>MALLNFQKPDKVIMIDSTDFEGKFEFRPLEPGYGLTVGNALRRVLLSSLEGFAITSVRIDGVEHEFSVVPGVVEDVTEIILNLKQVRFKRQIDDVESETVSISVSGKEQLTAGDFQKFISGYQVLNPDLVICNMGPKVSINMEIVIEKGRGYVPAEENKKSNAPLGSIAVDSVYTPVKNVKYSIENYRVEQKTDYEKLVFEIITDGSIHPKDALTEAAKVLIHHFMLFSDERITLEADEIAQTETYDEESLHMRQLLKTKLVDMDLSVRALNCLKAAEVDTLGDLVSFNKNDLMKFRNFGKKSLTELEELVINKGLQFGMDLSKYKLDKD[2x];> MFTNTIERVNFASAKNIPEYPDFLDIQIKSFQDFFQLETKSDERGNEGLYNTFMENFPITDTRNQFVLEFLDYFIDPPRYSIQECIERGLTYSVPLKARLKLYCTDPEHEDFETIVQDVYLGTIPYMTPSGTFVINGAERVVVSQLHRSPGVFFGQSFHANGTKLYSARVIPFKGSWIEFATDINGVMYAYIDRKKKLPVTTLFRAIGFERDKDILEIFDLSEEVKVSKAGLKKVLGRKLAARVLNTWHEDFVDEDTGEVVSIERNEIILDRDTILEKEHIDEIIDADVKTILLHKENNAQSDYAIIHNTLQKDPTNSEKEAVEHIYRQLRNAEPPDEETARGIIEKLFFSDQRYSLGEVGRYRMNKKLGLDIGMDKEVLTKEDIITIIKYLIELINSKAEIDDIDHLSNRRVRTVGEQLSQQFGVGLARMARTIRERMNVRDNEVFTPIDLINAKTLSSVINSFFGTNQLSQFMDQTNPLAEITHKRRLSALGPGGLSRERAGFEVRDVHYTHYGRLCPIETPEGPNIGLISSLSVFAKVNSMGFLETPYRKVVDGKVDVKEHIYLSAEEEEGMKIAQANIPLKDDGTIDREKVIARDEGDFPVVDPVEINYTDVAPNQIASISASLIPFLEHDDANRALMGSNMMRQAVPLLRPESPIVGTGLERQVATDSRVLINAEGDGVVEYVDAQKITIKYDRTEEERLVSFEEDSKTYELVKFRKTNQGTSINLKPIVRKGDKVKKGQVLCEGYATEKGELALGRNMKVAFMPWKGYNFEDAIVISEKVVREDIFTSVHIDEYALEVRDTKLGAEELTNDIPNVSEEATRDLDEYGMIRIGAEVKPGDILIGKITPKGESDPTPEEKLLRAIFGDKAGDVKDASLKASPSLRGVVIDKKLFSRSIKDKRKRSEDKEAISRLEMDYEVKFQQLKDVLIEKLFGLVNGKTSQGVINDLGEEVLPKGKKYTIKMLNAVDDFAHLVGGSWTTDEDTNALVADLLHNYKIKLNDIQGNLRRDKFTISVGDELPAGIMKLAKVYIAKKRKLKVGDKMAGRHGNKGIVARIVRQEDMPFLEDGTPVDIVLNPLGVPSRMNIGQIYETVLGWAGLKLGQKYGTPIFDGATLDDINELTDKAGVPRFGHTYLYDGGTGQRFDQAATVGVIYMLKLGHMVDDKMHARSIGPYSLITQQPLGGKAQFGGQRFGEMEVWALEAYGASATLREILTVKSDDVIGRAKTYESIVKGETMPEPGLPESFNVLMHELKGLGLDIRLEE;> MARIKDNNAPKRFNKISIGLASPESILAESRGEVLKPETINYRTHKPERDGLFCERIFGPVKDYECACGKYKRIRYRGIVCDRCGVEVTEKKVRRDRVGHINLVVPVAHIWYFRSLPNKIGYLLGLPSKKLDMIIYYERYVVIQPGIAKGPEGEEIHKLDFLTEEEYLNILESLPSENQYLEENDPNKFIAKMGAECLIDLLARIDLEQLSYELRHKANTETSKQRKTEALKRLQVVEALRESQDNRENNPEWMIMKVIPVIPPELRPLVPLDGGRFATSDLNDLYRRVIIRNNRLKRLMEIKAPEVILRNEKRMLQEAVDSLFDNTRKASAVKTESNRPLKSLSDSLKGKQGRFRQNLLGKRVDYSARSVIVVGPEMKLYECGLPKDMAAELYKPFIIRKLIERGIVKTVKSAKKIIDKKEPVVWDILENVLKGHPVLLNRAPTLHRLGIQAFQPKLIEGKAIRLHPLACTAFNADFDGDQMAVHLPLGPEAILEAQLLMLASQNILNPANGSPITVPSQDMVLGLYYMTKEKRSTPEEPVIGEGLTFYSSEEVEIAFNERKVALNAIIKVRTKDFNEAGELVNKIIETTVGRVLFNTVVPEQAGYINTVLNKKSLRNIIGDILAVTDVPTTADFLDKIKTMGYEFAFKGGLSFSLGDIIIPKEKHEMIAEANEQVDGIMMNYNMGLITFNERYNQVIDVWTSTNAMLTELAMKRIREDKQGFNSVYMMLDSGARGSKEQIRQLTGMRGLMAKPKKSTAGGGEIIENPI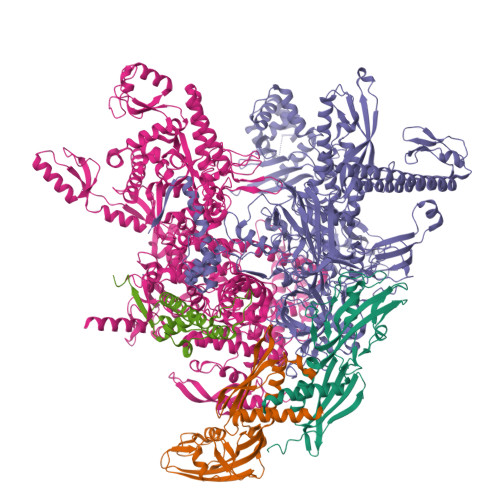LSNFKEGLSILEYFISTHGARKGLADTALKTADAGYLTRRLVDVSQDVIINTEDCGTLRGIEVEALKKNEEVVETLGERILGRVSLHDVYNPLTEELILKAGQEISEADVKKVEAAPIEKVEVRSPLTCEAAQGICAKCYGRNLATNKMVQRGEAVGVVAAQSIGEPGTQLTLRTFHVGGIAGNISEDSKLEAKFDGIAEIEDLRVVEGVDNGGGKSDIVISRTSEIKIVDAKTGITLSTNNIPYGSQLFVKNGEKITKGTVICQWDPYNGVIVSEFTGQIAYENIEQGMTYQVEIDEQTGFQEKVISESRNKRLIPTLLIKDGKGETIRSYNLPVGSHLMVDNGEKIKEGKILVKIPRKSAKAGDITGGLPRVTELFEARNPSNPAVVTEIDGVVSFGKIKRGNREIIIESKAGEVKKYLVKLSNQILVQENDYVRAGMALSDGSITPEDILAIKGPSAVQQYLVNEVQEVYRLQGVKINDKHFEVVVRQMMRKVQIQDSGDTTFLENQLVHKDDFINENDEIFGKKVVEDAGDSERLKPGQIVTARQLRDENSILRREDKTLVTARDAVAATATPILQGITRASLQTKSFISAASFQETTKVLNEAAVNGKVDTLEGLKENVIVGHKIPAGTGMRDYDSIIVGSKEEYDEIMARKEEFKF;> MQDLKNTKAPVSTATLNRNEFDSKTGNIYEAISIASKRAVQINSDIKKELLEKLEEFATYSDSLEEVFENKEQIEVSKFYEKLPKPHALAVQEWLEDKIYYRNTEKDA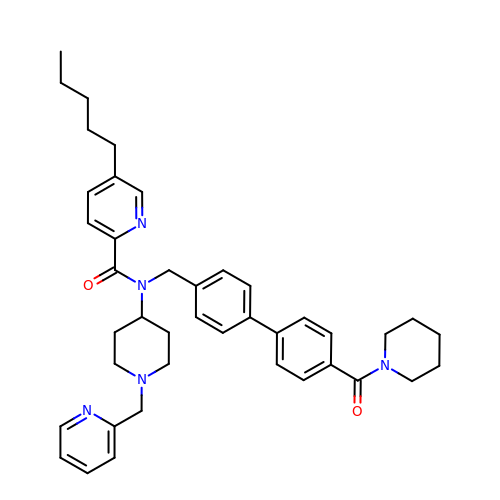5-PENTYL-N-{[4'-(PIPERIDIN-1-YLCARBONYL)BIPHENYL-4-YL]METHYL}-N-[1-(PYRIDIN-2-YLMETHYL)PIPERIDIN-4-YL]PYRIDINE-2-CARBOXAMIDE | C41 H49 N5 O2 | RBZSSVVTHOATHE-UHFFFAOYSA-N FLUORO-PHOSPHITE 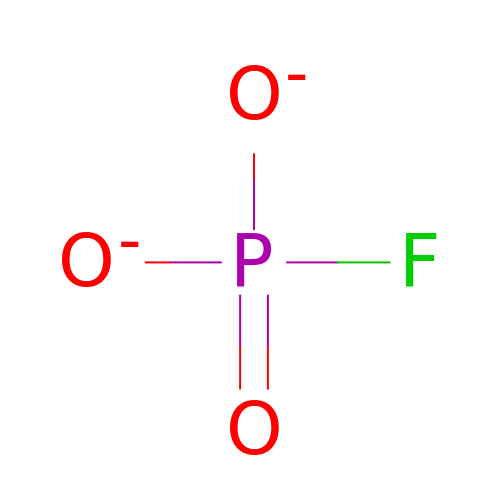ION | F O3 P | DWYMPOCYEZONEA-UHFFFAOYSA-L> SNAMARTRSADYENIRD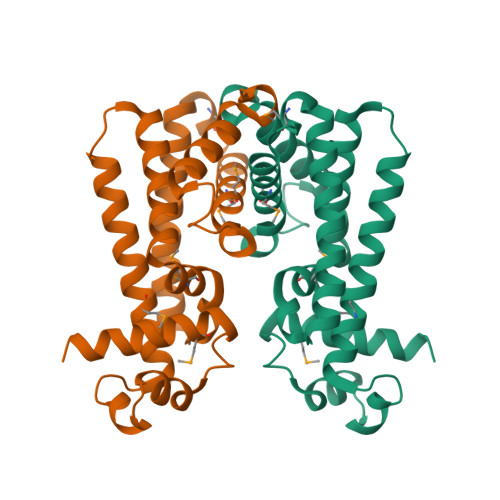TIIERAAAMFARQGYSETSIGDIARACECSKSRLYHYFDSKEAVLRDMLTTHVDSLLERCRQVLYGSNEPKTRFLQIVKLFLEIYATSRDRHVVMLTCLDALPEDQRKALIAKQRELIAYVRDALLQLRPDMAANRTLAHVDTMLFFGMINWTYTWYKADGSVSPDALAERTVQLFLDGYLNLLSA>[2x]MAEAGLRGWLLWALLLRLAQSEPYTTIHQPGYCAFYDECGKNPELSGSLMTLSNVSCLSNTPARKITGDHLILLQKICPRLYTGPNTQACCSAKQLVSLEASLSITKALLTRCPACSDNFVNLHCHNTCSPNQSLFINVTRVAQLGAGQLPAVVAYEAFYQHSFAEQSYDSCSRVRVPAAATLAVGTMCGVYGSALCNAQRWLNFQGDTGNGLAPLDITFHLLEPGQAVGSGIQPLNEGVARCNESQGDDVATCSCQDCAASCPAIARPQALDSTFYLGQMPGSLVLIIILCSVFAVVTILLVGFRVAPARDKSKMVDPKKGTSLSDKLSFSTHTLLGQFFQGWGTWVASWPLTILVLSVIPVVALAAGLVFTELTTDPVELWSAPNSQARSEKAFHDQHFGPFFRTNQVILTAPNRSSYRYDSLLLGPKNFSGILDLDLLLELLELQERLRHLQVWSPEAQRNISLQDICYAPLNPDNTSLYDCCINSLLQYFQNNRTLLLLTANQTLMGQTSQVDWKDHFLYCANAPLTFKDGTALALSCMADYGAPVFPFLAIGGYKGKDYSEAEALIMTFSLNNYPAGDPRLAQAKLWEEAFLEEMRAFQRRMAGMFQVTFMAERSLEDEINRTTAEDLPIFATSYIVIFLYISLALGSYSSWSRVMVDSKATLGLGGVAVVLGAVMAAMGFFSYLGIRSSLVILQVVPFLVLSVGADNIFIFVLEYQRLPRRPGEPREVHIGRALGRVAPSMLLCSLSEAICFFLGALTPMPAVRTFALTSGLAVILDFLLQMSAFVALLSLDSKRQEASRLDVCCCVKPQELPPPGQGEGLLLGFFQ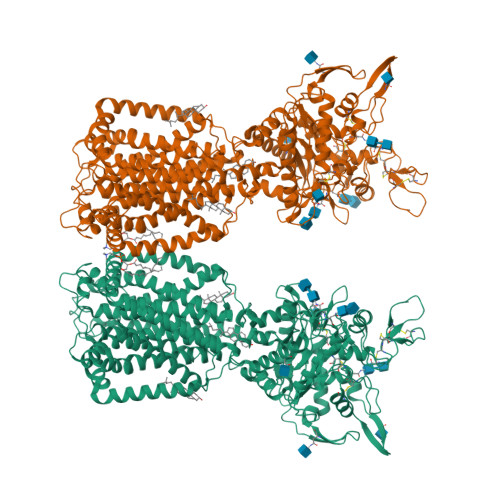KAYAPFLLHWITRGVVLLLFLALFGVSLYSMCHISVGLDQELALPKDSYLLDYFLFLNRYFEVGAPVYFVTTLGYNFSSEAGMNAICSSAGCNNFSFTQKIQYATEFPEQSYLAIPASSWVDDFIDWLTPSSCCRLYISGPNKDKFCPSTVNSLNCLKNCMSITMGSVRPSVEQFHKYLPWFLNDRPNIKCPKGGLAAYSTSVNLTSDGQVLTSRFMAYHKPLKNSQDYTEALRAARELAANITADLRKVPGTDPAFEVFPYTITNVFYEQYLTILPEGLFMLSLCLVPTFAVSCLLLGLDLRSGLLNLLSIVMILVDTVGFMALWGISYNAVSLINLVSAVGMSVEFVSHITRSFAISTKPTWLERAKEATISMGSAVFAGVAMTNLPGILVLGLAKAQLIQIFFFRLNLLITLLGLLHGLVFLPVILSYVGPDVNPALALEQKRAEEAVAAVMVASCPNHPSRVSTADNIYVNHSFEGSIKGAGAISNFLPNNGRQF> XATAAA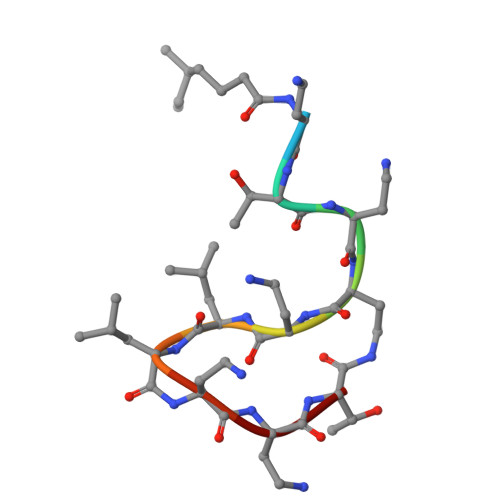LLAAT> ATLRTVGDLTWLNVSTTDVGKWIRVENRHGKGECFVTATDVGTWCSDSVGYECPQIAPAYDPEDLDCYCRNTSTYVTYGRCKNGRSGRSRSKRAITIAPHGEAGLRVGSTKHWTSRATPQRYLMRVEKWVLRHPLPA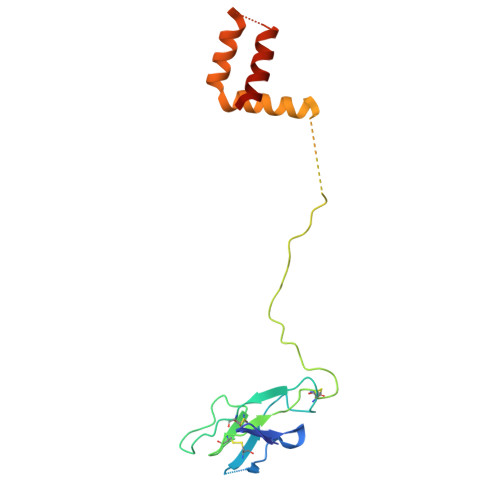LVLVVLGWMMGRSHGQRAMYIVLMLLVAPSYG> NAAVHLTLK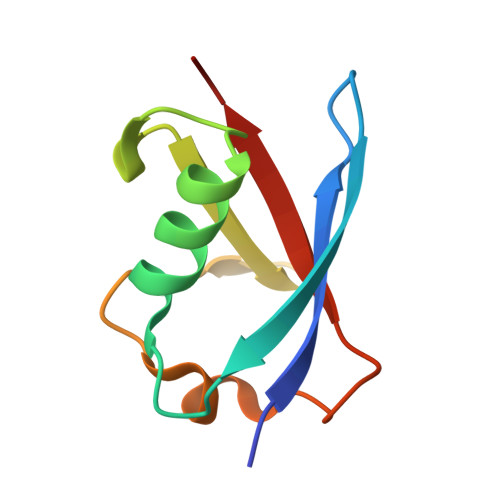KIQAPKFSIEHDFSPSDTILQIKQHLISEEKASHISEIKLLLKGKVLHDNLFLSDLKVTPANSTITVMIKPN We reconstituted the biosynthesis of the benzoxazole moiety found in nataxazole by adding two enzymes (NatL2, NatAM), to 3‐HAA, ATP, and Mg2+. We have determined the structures of both NatL2 (homologue of BomJ) and NatAM (homologue of BomN) from the antitumor nataxazole pathway. We show NatL2 catalyzes ester not, as previously reported, amide formation; the amide is a shunt product. NatAM catalyzes benzoxazole from this ester by a mechanism that we propose involves shuttling of protons to control the fate of a hemiorthoamide intermediate.

We therefore soaked the co‐crystallized AMP:3HAA crystals with salicylic acid (SA), which lacks the hydroxyl at the meta position. In subunit A, two molecules of SA are bound but no AMP. One SA molecule, denoted SA1 has replaced 3‐HAA1. and occupies the same pocket with differences in orientation. A second molecule of SA, denoted SA2 is unambiguously located where we had tentatively identified 3‐HAA2. The pocket is formed by Thr128, Ala211, Ala212, Thr135, and Trp178. The carboxylate of SA2 makes a salt bridge with Arg156 that orients the molecule. A simple in silico change of the SA2 molecule to 3‐HAA2 molecule and combination with the 3‐HAA1‐AMP adenylate allows creation a model for the second reaction, the attack of hydroxyl (not the amine) of 3‐HAA2 upon the 3‐HAA1‐adenylate to yield the ester (not the amide). SA, which lacks a hydroxyl group at the meta position, gives no reaction, indicating that the hydroxyl must be at the meta position for reaction.

> MSRSRPELGDWSSPAELAELQRSQLPRVLAQALRSPFYAARYRGTTPPRTADDFAGVEVTAKQDLRDQYPFGMLAVGREHLATYHESSGTAGEPTASYYTEEDWTDLAERFARKWTGIHPSDTFLVRTPYGLVITGHLAQAAGRLRGATVVPGDARSLATPLSRMVRVLKTLDVTLTWCNPTEITMLAAAAKAAGLRPDQDFPHLRAMFTAAEPLTEVRRRRLSEIWGGIPVVEEYGSTETGTIAGQCPEGRMHLWADRAIFEVYDPRTGTLSEAGRGQMVVTPLYRDAMPLLRYNLADDVEVSTDPCGCGWLLPTVTVLGRAGTGHRIGPATVTQQRLEELVFSLPAAYEVMFWRAKAHPDVLELEFEAPEPVRQRAVKELGAALDRELGVPHRITGLAPGTLVPAEALTAQRDILKARYLFAEDEDWDKAVMYF;> AMSRSRPELGDWSSPAELAELQRSQLPRVLAQALRSPFYAARYRGTTPPRTADDFAGVEVTAKQDLRDQYPFGMLAVGREHLATYHESSGTAGEPTASYYTEEDWTDLAERFARKWTGIHPSDTFLVRTPYGLVITGHLAQAAGRLRGATVVPGDARSLATPLSRMVRVLKTLDVTLTWCNPTEITMLAAAAKAAGLRPDQDFPHLRAMFTAAEPLTEVRRRRLSEIWGGIPVVEEYGSTETGTIAGQCPEGRMHLWADRAIFEVYDPRTGTLSEAGRGQMVVTPLYRDAMPLLRYNLADDVEVSTDPCGCGWLLPTVTVLGRAGTGHRIGPATVTQQRLEELVFSLPAAYEVMFWRAKAHPDVLELEFEAPEPVRQRAVKELGAALDRELGVPHRITGLAPGTLVPAEALTAQRDILKARYLFAEDEDWDKAVMYF>[6x]MGQKDSAPAASASAAADNGAA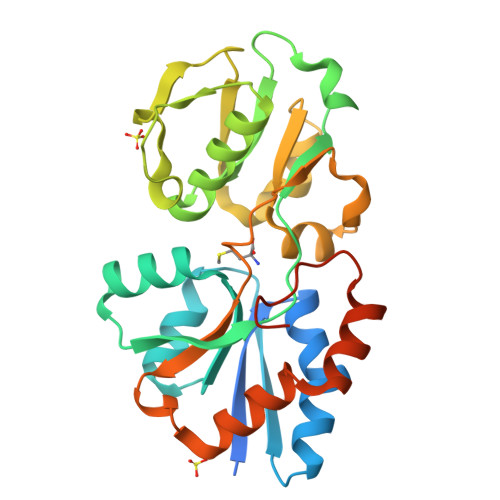KKEIVFGTTVGDFGDMVKEQIQPELEKKGYTVKLVEFTDYVRPNLALAEGELDINVFQHKPYLDDFKKEHNLDITEVFQVPTAPLGLYPGKLKSLEEVKDGSTVSAPNDPSNFARVLVMLDELGWIKLKDGINPLTASKADIAENLKNIKIVELEAAQLPRSRADVDFAVVNGNYAISSGMKLTEALFQEPSFAYVNWSAVKTADKDSQWLKDVTEAYNSDAFKAYAHKRFEGYKSPAAWNEGAAKLEHHHHHH> MGGSHHHHHHGMASLENLYFQADQPIDADVTVIGSGPGGYVAAIKAAQLGFKTVCIEKNETL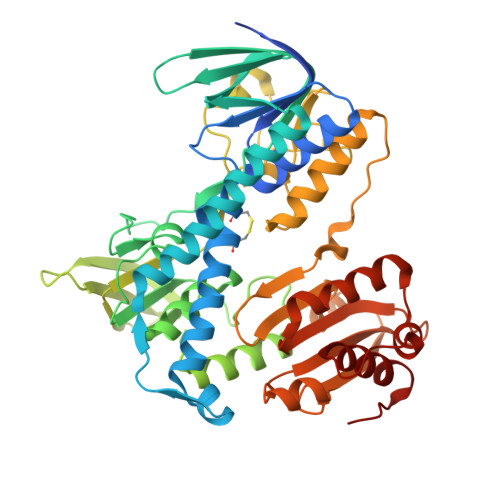GGTCLNVGCIPSKALLNNSHYYHMAHGKDFASRGIEMSEVRLNLDKMMEQKSTAVKALTGGIAHLFKQNKVVHVNGYGKITGKNQVTATKADGGTQVIDTKNILIATGSEVTPFPGITIDEDTIVSSTGALSLKKVPEKMVVIGAGVIGVELGSVWQRLGADVTAVEFLGHVGGVGIDMEISKNFQRILQKQGFKFKLNTKVTGATKKSDGKIDVSIEAASGGKAEVITCDVLLVCIGRRPFTKNLGLEELGIELDPRGRIPVNTRFQTKIPNIYAIGDVVAGPMLAHKAEDEGIICVEGMAGGAVHIDYNCVPSVIYTHPEVAWVGKSEEQLKEEGIEYKVGKFPFAANSRAKTNADTDGMVKILGQKSTDRVLGAHILGPGAGEMVNEAALALEYGASCEDIARVCHAHPTLSEAFREANLAASFGKSINF>PHEELQYLRQLREILCRGSDRLDRTGIGTLSLFGMQARYSLRDHFPLLTTKRVFWRGVVQELLWFLKGSTDSRELSRTGVKIWDKNGSREFLAGRGLAHRREGDLGPVYGFQWRHFGAAYVDADADYTGQGFDQLSYIVDLIKNNPHDRRIIMCAWNPADLSLMALPPCHLLCQF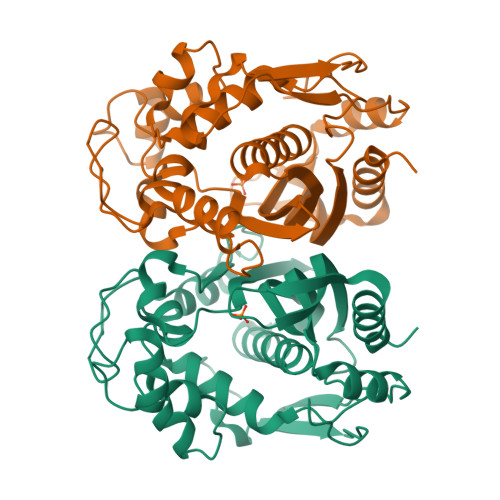YVADGELSCQLYQRSGDMGLGVPFNIASYSLLTYMLAHVTGLRPGEFIHTLGDAHIYKTHIEPLRLQLTRTPRPFPRLEILRSVSSMEEFTPDDFRLVDYCPHPTIRME[2x]>[2x]MTTQPLNSHRVDPHTAQKFYIDGHWSAPLSPVSIAVVNPATEEVVAHVASGSAADVDRAVAAARAAFAGWSGTSPEVRAQVIGRIHELIIERKEELAQAISLEMGAAISSARAMQVPLAAEHVRVARDLLATYRFQTVEGGTAIEREPIGVCALITPWNWPLYQITAKVAPAIAAGCTVVLKPSELSPLSAL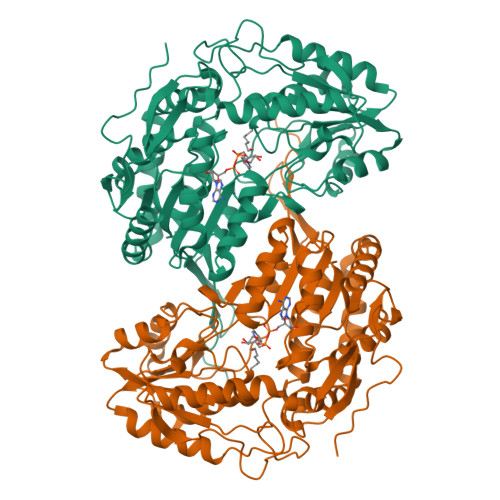LFAQLVHDAGLPPGVFNLVNGSGPEVGGAMAAHPDIDMISITGSNRAGALVAQAAAPTVKRVTQELGGKSPNILLPDADFANAVPPGVMAAFRNVGQSASAPTRMIVPRNRLAEVEALAAQTAGTIVVGDPQLEHTVLGPIANEAQFHRVQAMINAGICEGAKLVCGGPGRVQGHEQGFYTRPTVFSEVDSSMRIAREEIFGPVLCLIAYDTIDEAVAIANDTVYGLGAHVQGQDLELARSVASRIRAGQVHLNYPSWNPMAPFGGYKRSGNGREYGVHGFEEYLETKAIVGFAPADLM> MFDSLSPQELAALHARHQQDYAALQGMKLALDLTRGKPSAEQLDLSNQLLSLPGDDYRDPEGTDTRNYGGQHGLPGLRAIFAELLGIAVPNL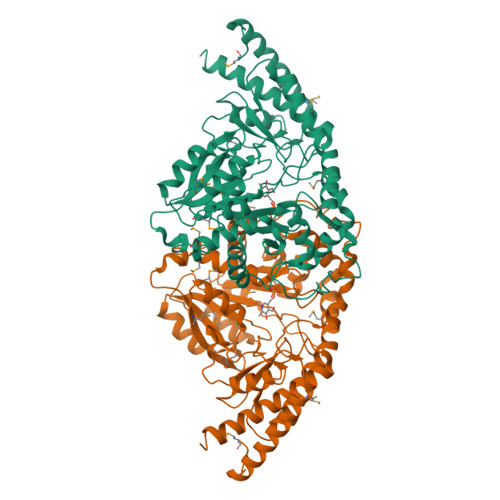IAGNNSSLELMHDIVAFSMLYGGVDSPRPWIQEQDGIKFLCPVPGYDRHFAITETMGIEMIPIPMLQDGPDVDLIEELVAVDPAIKGMWTVPVFGNPSGVTYSWETVRRLVQMRTAAPDFRLFWDNAYAVHTLTLDFPRQVDVLGLAAKAGNPNRPYVFASTSKITFAGGGVSFFGGSLGNIAWYLQYAGKKSIGPDKVNQLRHLRFFGDADGVRLHMLRHQQILAPKFALVAEVLDQRLSESKIASWTEPKGGYFISLDVLPGTARRTVALAKDVGIAVTEAGASFPYRKDPDDKNIRIAPSFPSVPDLRNAVDGLATCALLAATETLLNQGLASSHHHHHH>[6x]MKIKTLAIVVLSALSLSSTAALAAATTVNGGTVHFKGEVVNAACAVDAGSVDQTVQLGQVRTASLAQEGATSSAVGFNIQLNDCDTNVASKAAVAFLGTAIDAGHTNVLALQSSAAGSATNVGVQILDRTGAALTLDGATFSSETTLNNGTNTIPFQARYFATGAATPGAANADATFKVQYQ

Type 1 pili are important virulence factors of uropathogenic Escherichia coli that mediate bacterial attachment to epithelial cells in the urinary tract. The pilus rod is comprised of thousands of copies of the main structural subunit FimA and is assembled in vivo by the assembly platform FimD. The pilus rod is a right-handed superhelical structure composed of ~3.2 subunits per turn with an axial rise between two consecutive subunits of 7.8 Å or 7.7 Å for the type 1 and P pilus rods, respectively. All subunits in the rod are connected via DSE, forming an exceptionally stable fold that is resistant to extreme temperatures, denaturants and mechanical stress.

To investigate whether FimD is responsible for the increased stability of in vivo-assembled pili, we assembled FimD-catalysed pili in vitro (hereafter denoted as FimD-cat) in a reaction where FimDCH was primed by the addition of FimC–FimF. The resulting unfolding half-lives (t½) at 6.45 M GdmCl showed that the FimD-cat pili (t½ = ~1700 s) were almost as stable as the in vivo-assembled pili (t½ = ~19,800 s) and significantly more stable than pili assembled in vitro (t½ = 26 s) at 6.45 M GdmCl. Moreover, the dependence of the unfolding half-life on GdmCl of FimD-cat pili also displayed the same characteristic kink at high GdmCl concentrations as that of in vivo-assembled pili (>6.75 M). The melting temperature of in vitro-assembled pili was significantly lower (59 °C) than for pilus samples assembled in vivo (79 °C) or in the presence of FimD (78 °C). Importantly, the stability of in vitro-assembled type 1 pilus rods can be restored to near-in vivo levels by the addition of FimD to the assembly reaction. Our structures of in vivo-assembled, in vitro-assembled and FimD-cat pilus rods were resolved to 2.85, 2.69 and 2.52 Å, respectively. We modelled six adjacent FimA subunits linked through donor-strand interactions and refined the models against their respective cryo-EM maps. The Cα root mean square deviation (RMSD) from global alignment of the three models was less than 1 Å in each case (0.68 Å, 0.69 Å and 0.25 Å for FimD-cat vs. in vivo, FimD-cat vs. in vitro and in vitro vs. in vivo, respectively) implying that all three structures are highly similar. More detailed analyses did not show any significant differences in residue contacts or subunit–subunit interfaces between all three models.> LRPVLPTQSAHDPP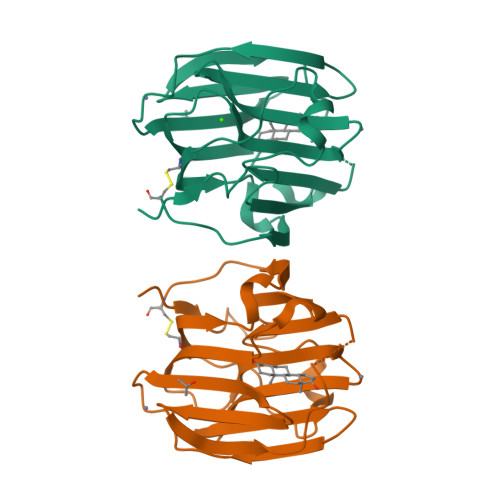AVHLSNGPGQEPIAVMTFDLTKITKTSSSFEVRTWDPEGVIFYGDTNPKDDWFMLGLRDGRPEIQLHNHWAQLTVGAGPRLDDGRWHQVEVKMEGDSVLLEVDGEEVLRLRQVSGPLTSKRHPIMRIALGGLLFPASNLRLPLVPALDGCLRRDSWLDKQAEISASAPTSLRSCDVESNPGIFLPPGTQAE> MNDFLFYLDIFGVIVFALSGALMAGRYQLDPFGVVVLASVTAVGGGTIRDVILQTPVFWVEKPYYLYVILATAILTIVLIRQPKRIPKRFLLIADALGLALFAVLGTQKALYLGAPIPVAVVLGTITGIAGGMIRDVLCNVIPMILREEIYALAAMLGGSLFIILHGLNWNDTNAMIVSISAALALRLAAIYW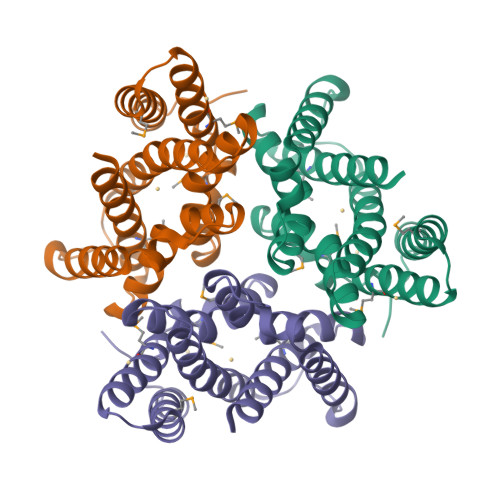HVSLPAFHIVEKPKKEKGTTKIIEKKAAAENLYFQGLEDYKDDDDKHHHHHHHHHH>[4x]GPGSGPRPAQLTWSQLPEVLESGVLDTLSTEERKRQEAIFEILTSEFSYLHSLSILVTEFLQSRELRATMTQTEHHHLFSNILDVMSASQKFFEALEQRHKAQVCVEDISDILEDHAQHHFHPYIAYC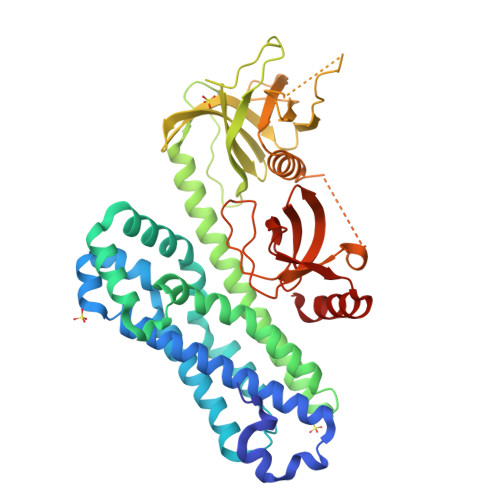SNEVYQQRTLQKLSNSNAAFRDVLKEIEKRPACGGLPMISFLILPMQRVTRLPLLTDTLCLKTQGHPERYKAASQALKAISKLVKQCNEGAHKMERTEQIYTLNMQLDFGKVKSLPLISASRWLLKRGELFLLEESSIFRKIASRPTCYLFLFNDVLVVTKKKSEESYLVQDYAQLDHVQVRKLEPSEPLLPGGSSRSSSVPYPFQVNLLHNSEGRQEQILLSSDSASDRARWITALTYKERQWQGITNKGELPQVEVTKAYFAKQADEITLQQADIVLVLQEEDGWLHGERLRDGETGWFPESFAHSITSRVAVEGNVRRMERLRVETDV>[3x]MGSGMEWFPLLGLANRARK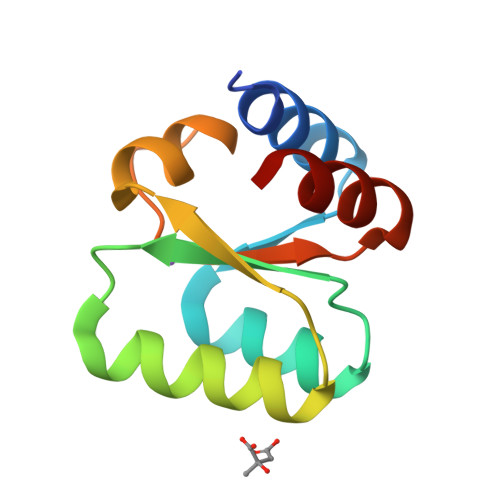VVSGEDLVIKEIRNARAKLVLLTEDASSNTAKKVTDKCNYYKVPYKKVESRAVLGRSIGKEARVVVAVTDQGFANKLISLLD> GAACGACACAGA;> CGGCGACTC;> TCTCCG;>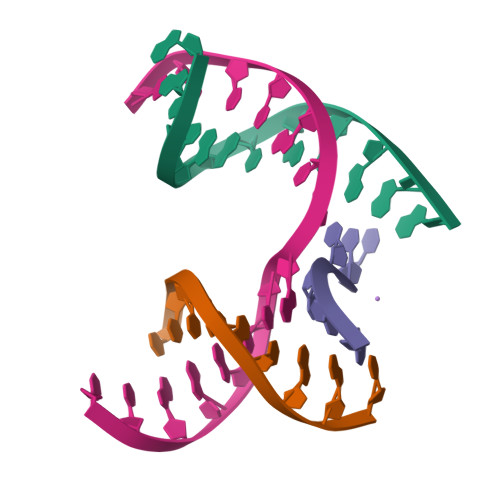 TCGAGTCGGTGTCGT> MKESLKDRIRLWKRLYVNAFENALNAIPNVKGVLLAYNTNIDAIKYLDKDDLEKRVTEIGKEKVFEIIENPPEKISSIEELLGGILRSIKLGKAMEWFVESEEVRRYLREWGWDELRIGGQAGIMANLLGGVYRIPTIVHVPQNPKLQAELFVDGPIYVPVFEGNKLKLVHPKDAIAEEEELIHYIYEFPRGFQVFDVQAPRENRFIANADDYNARVYMRREFREGFEEIT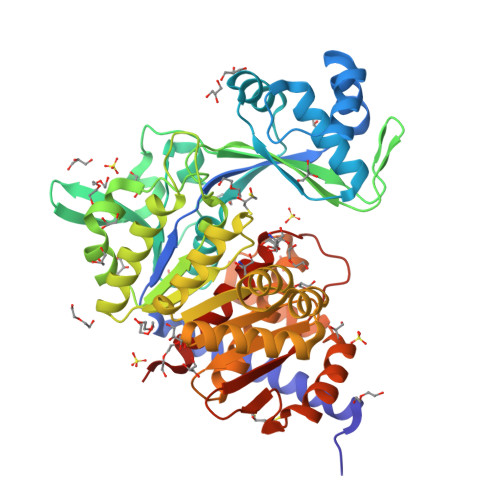RNVELAIISGLQVLKEYYPDGTTYRDVLDRVESHLNILNRYNVKSHFEFAYTANRRVREALVELLPKFTSVGLNEVELASIMEIIGDEELAKEVLEGHIFSVIDAMNVLMDETGIERIHFHTYGYYLALTQYRGEEVRDALLFASLAAAAKAMKGNLERIEQIRDALSVPTNERAIVLEEELEKEFTEFENGLIDMVDRQLAFVPTKIVASPKSTVGIGDTISSSAFVSEFGMRKR3-(2-BENZOTHIAZOLYLTHIO)-1-PROPANESULFONIC 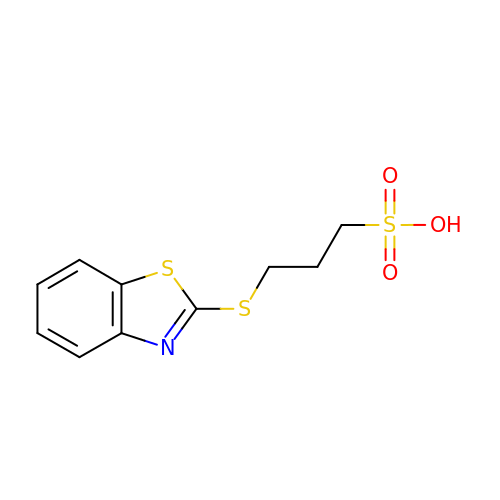ACID | C10 H11 N O3 S3 | XBNHRNFODJOFRU-UHFFFAOYSA-N> MAYRALMVLRMDPADAEHVAAAFAEHDTTELPLEIGVRRRVLFRFHDLYMHLIEA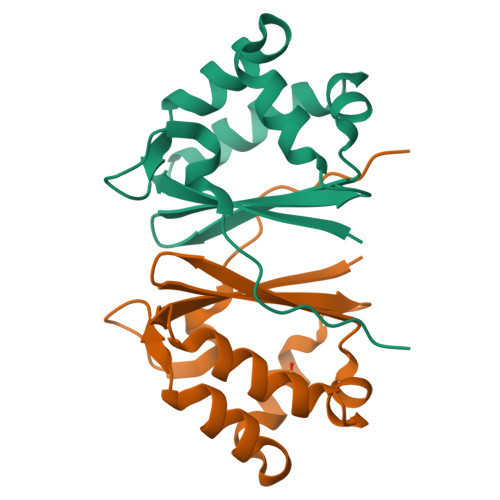DDDIMERLYQARSHPLFQEVNERVGQYLTPYAQDWEELKDSKAEVFYSWTAPDS In this work, we report the identification of an O2-sensitive isethionate sulfo-lyase, which catalyzes C–S cleavage of isethionate via a radical-dependent mechanism. GREs catalyze challenging chemical transformations using the high reactivity of the protein-based radical to initiate catalytic reactions, and recent studies have yielded several new GREs with novel catalytic chemistry. The essential O2-sensitive glycyl radical (G•) cofactor is generated by an activating enzyme through chemistry involving S-adenosylmethionine (SAM) and a [4Fe-4S]1+ cluster. Biochemical characterization confirmed that GUF was indeed an isethionate sulfo-lyase (vide infra), and we renamed GUF and its activating enzyme IseG and IseH, respectively.

To further investigate the mechanism of C–S cleavage by IseG, we determined the crystal structure of isethionate-bound IseG at 2.4 Å. The P21 crystals contain four monomers per asymmetric unit, each exhibiting a canonical β/α barrel fold common to other GREs. The sulfonate group of isethionate is coordinated by Arg187, Gln191, and Arg676 of IseG and one water molecule through an extensive hydrogen bond network. The conformation of isethionate is further stabilized by van der waals contact with Phe680, Ile190, and Thr310. The three sulfonate-coordinating residues (Arg187, Gln191, and Arg676) are conserved in the sequences within the “IseG” cluster of the GRE SSN, but are absent in CutC and other GREs, supporting the proposal that the “IseG” cluster enzymes are involved in sulfonate degradation. Despite overall structural similarities between IseG and CutC, two substrate-interacting loops (loop A and B) in IseG are shifted by up to 6.8 Å relative to CutC, resulting in dramatic changes to the binding pocket structure and substrate-coordinating residues. The orientation of the isethionate C2 and sulfonate-leaving group differs greatly from choline in CutC. A 98.5° rotation of the C1–C2 axis in isethionate vs. choline results in the pro-R hydrogen of isethionate being oriented for abstraction by the thiyl radical. Incubation of activated IseG with isethionate resulted in its conversion to acetaldehyde and sulfite.

>SNARYRATHERVFTILESFDNTRPRIDVERAKYFTESMKATEGQPLPLRWAKALMHIAENMTVYIDDHQLICGRAGYQGRYGVLYPELDGDFLGTAIEDLPNRAESPFAITPAAAAVVVEEIAPFWKGKTYHEALNLALPADVHKLTYDDPQGLMSRFIVNETSSFRSSIQWVHDYEKVLKRGFRSIKEEALEKIAALDPMSPCDNVEKRPFLEAIVIVCDAIILWAKRHAKLAAELAAKETDPTRKRELETMAEICAWVPENPARTFHEAVQAQWFTQVFSRIEQKTGTIVSNGRMDQYFWPFYEKDLAEGRITEDSALELLECMWVGMAQYVDLYISPTGGAFNEGYAHWEAVTIGGQTPEGRDATNDLTYLFLKSKREFPLHYPDLAARIHSRSPERYLWEVAETIKDGSGFPKLINDEEVVPLYVSKGATFAEALDYAVSGCTEARMPNRDTYTSGGAYINFAAALEMVLYNGKMLKYGDTDLGAHTGDPCEFKTWEEFWNAYVTQHHLFLKTAFVQQHIINNLRARHFAQPMGSSLHDLCMKHCLDLHTPQIPEGINLGYFEYMGFGTVVDSLSAIKKLVFEDKKLTMGELIEALKCNFEGKEDIQQLLKSAPCYGNNDDYADSIARDIDALSVKYGRRYSPELGMHNDVRYVPFTSHVPFGRVVSATPNGRKAWSALSDGSSASHGADVNGPTAILQSNFNSKNYGMRDRAARMLNIKFTPKCVEGEEGSQKLVSFIRTFCDLKLWHVQFNVINKETLLAAQRDPEKYRNLIVRIAGYSAYFVDLSPDLQNDLIARTGHDVM[4x]>[2x]RERRFTSDAAHELRSPLTALKVQTEVAQLSDDDPQARKKALLQLHSGID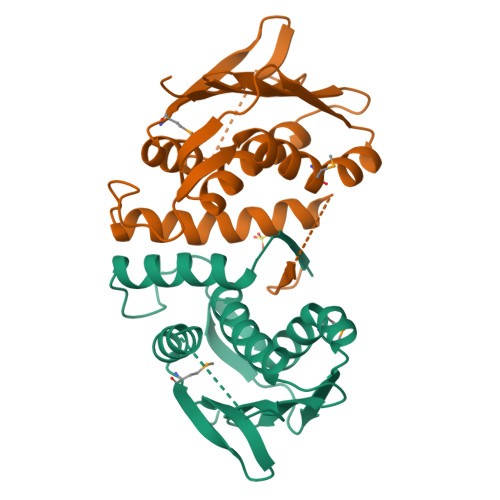RATRLVDQLLTLSRLDSLDNLQDVAEIPLEDLLQSSVMDIYHTAQQAKIDVRLTLNAHSIKRTGQPLLLSLLVRNLLDNAVRYSPQGSVVDVTLNADNFIVRDNGPGVTPEALARIGERFYRPPGQTATGSGLGLSIVQRIAKLHGMNVEFGNAEQGGFEAKVSWLEHHHHHH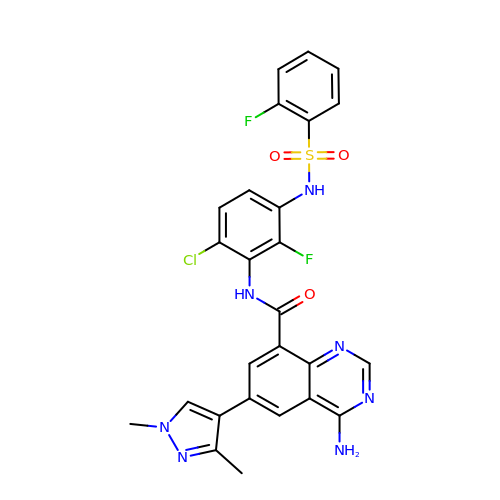4-amino-N-(6-chloro-2-fluoro-3-{[(2-fluorophenyl)sulfonyl]amino}phenyl)-6-(1,3-dimethyl-1H-pyrazol-4-yl)quinazoline-8-carboxamide | C26 H20 Cl F2 N7 O3 S | SLZQHMNLJFHHQH-UHFFFAOYSA-N> XSLSDKDKAAVRALWSKIGKSSDAIGNDALSRMIVVYPQTKIYFSHWPDVTPGSPNI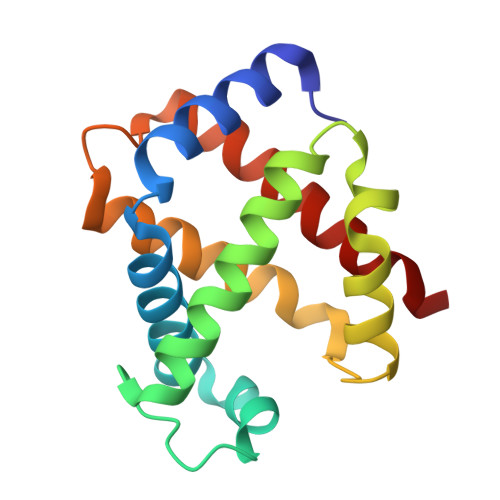KAHGKKVMGGIALAVSKIDDLKTGLMELSEQHAYKLRVDPSNFKILNHCILVVISTMFPKEFTPEAHVSLDKFLSGVALALAERYR>[4x]AGVAKFAKYPLTFGPSPISNLNRLSQHLGSKVNVYAKREDCNSGLAFGGNTLRKLEYIVPDIVEGDYTHLVSIGGRQSNQTRMVAALAAKLGKKCVLIQEDWVPIPEAEKDVYNRVGNIELSRIMGADVRVIEDGFDIGMRKSFANALQELEDAGHKPYPIPAGCSEHKYGGLGFVGFADEVINQEV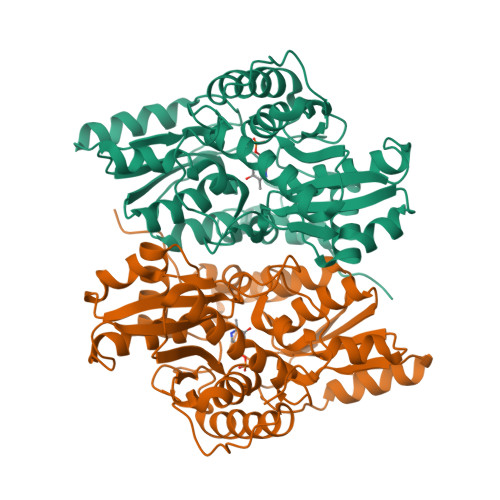ELGIKFDKIVVCCVTGSTTAGILAGMAQYGRQDDVIAIDASFTSEKTKEQTLRIANNTAKLIGVEHEFKDFTLDTRFAYPCYGVPNEGTIEAIRTCAEQEGVLTDPVYEGKSMQGLIALIKEDYFKPGANVLYVHLGGAPALSAYSSFFPTKTA URIDINE 3',5'-BIS(DIHYDROGEN 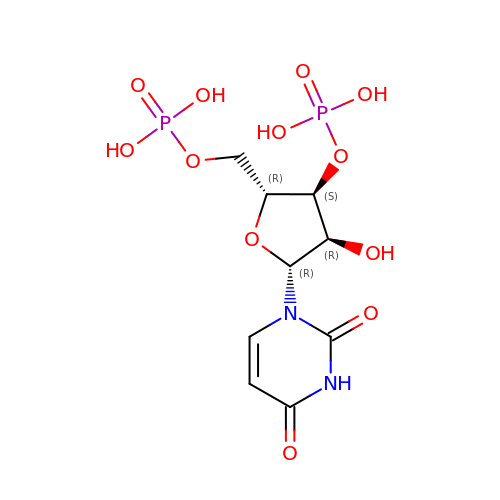PHOSPHATE) | C9 H14 N2 O12 P2 | ZPVPRWPOZBXDKD-XVFCMESISA-N>GPLGSISQNKRRYRKDGFDLDLTYVTDHVIAMSFPSSGRQSLFRNPIGEVSRFFKTKHPDKFRIYNLCSERGYDETKFDNHVYRVMIDDHNVPTLVDLLKFIDDAKVWMTSDPDHVIAIHCKAGKGRTGTLVSSWLLEDGKFDTAKEALEYFGSRRTDFEVGDVFQGVETASQIRYVGYFEKIKKNYGGQLPPMKKLKVTGVTITAIQGVGRGNGSDLSMQIVSERQEVLLCKFAEGYNCALQYDATDDCVTCEVKNCPVLAGDIKVRFMSTSKSLPRGYDNCPFYFWFNTSLVEGDHVTLKREEIDNPHKKKTWKIYRDNFTVKLTFSD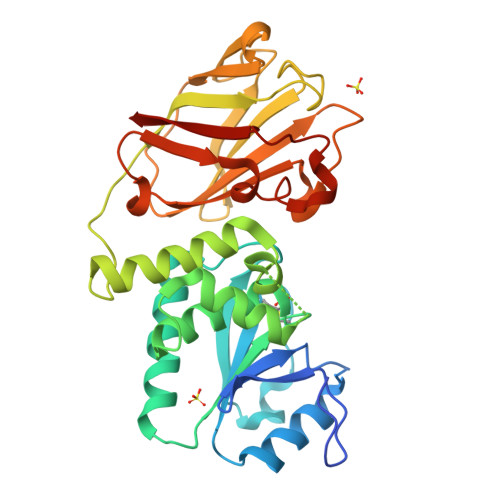AEDI[3x]> SVPIVSAWEKGMEAARALMDKYHVDNDLKANFKLLPDQVEALAAVCKTWLNEEHRGLQLTFTSNKTFVTMMGRFLQAYLQSFAEVTYKHHEPTGCALWLHRCAEIEGELKCLHGSIMINKEHVIEMDVTSENGQRALKEQSSKAKIVKNRWGRNVVQISNTDARCCVHDAACPANQFSGKSCGMFFSEGAKAQVAFKQIKAFMQALYPNAQTGHGH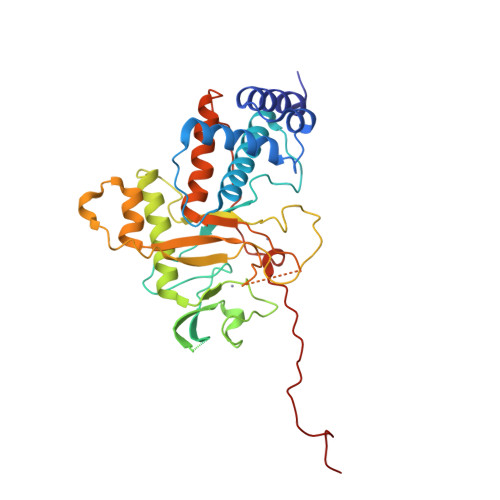LLMPLRCECNSKPGHAPFLGRQLPKLTPFALSNAEDLDADLISDKSVLASVHHPALIVFQCCNPVYRNSRAQGGGPNCDFKISAPDLLNALVMVRSLWSENFTELPRMVVPEFKWSTKHQYRNVSLPVAHSDARQNPFDF pmcHuman ornithine aminotransferase (hOAT) is an enzyme that catalyzes the transfer of the δ-amino group from l-ornithine (l-Orn) to α-ketoglutarate (α-KG). As a pyridoxal-5′-phosphate (PLP)–dependent transaminase, hOAT has a “Bi−Bi, Ping–Pong” kinetic mechanism. In the first half-reaction, PLP and l-Orn are converted to pyridoxamine phosphate (PMP) and l-glutamate-γ-semialdehyde (l-GSA). l-GSA is then prone to cyclize to Δ1-pyrroline-5-carboxylate (P5C). In the second half-reaction, hOAT catalyzes the transfer of the amino group of PMP to an α-keto acid, preferentially α-KG, forming glutamate and regenerating the PLP form of the cofactor.

To structurally assess the influence of low pH values, an X-ray crystal structure of hOAT at pH 6.0 was obtained with a resolution of 2.1 Å. After model building and refinements, the final model presents three monomers in an asymmetric unit of the C 1 2 1 space group. Although no major structural changes were detected in the overall quaternary and tertiary structure of hOAT at pH 6.0, some notable deviations were observed in local conformations of the active-site residues. Acidic conditions altered the position of the Arg180 side chain, a residue responsible for initial substrate recognition and binding. In addition, the side chain of Glu235 exhibited relatively weak electron density reflecting increased mobility of this residue at lower pHs. In the refined low pH model, the side chain of Glu235 faces away from Arg413. In the pH 6.0 structure, Arg180 moved toward the center of the active site occupying the space where the substrate would be localized. At pH 7.8, the distance between the two side chains is 7.8 Å, but it reduces to 5.7 Å at pH 6.0. This results in the constriction of the active-site pocket as shown in protein surface comparison in Figure 4C. The structure from hOAT crystallized at pH 6.0 revealed that the enzyme’s active site has rearranged side-chain conformations that hinder ligand entry to the catalytic pocket.

>[3x]MFSKLAHLQRFAVLSRGVHSSVASATSVATKKTVQGPPTSDDIFEREYKYGAHNYHPLPVALERGKGIYLWDVEGRKYFDFLSSYSAVNQGHCHPKIVNALKSQVDKLTLTSRAFYNNVLGEYEEYITKLFNYHKVLPMNTGVEAGETACKLARKWGYTVKGIQKYKAKIVFAAGNFWGRTLSAISSSTDPTSYDGFGPFMPGFDIIPYNDLPALERALQDPNVAAFMVEPIQGEAGVVVPDPGYLMGVRELCTRHQVLFIADEIQTGLARTGRWLAVDYENVRPDIVLLGKALSGGLYPVSAVLCDDDIMLTIKPGEHGSTYGGNPLGCRVAIAALEVLEEENLAENADKLGIILRNELMKLPSDVVTAVRGKGLLNAIVIKETKDWDAWKVCLRLRDNGLLAKPTHGDIIRFAPPLVIKEDELRESIEIINKTILSF> MAKEWGYASHNGPDHWHELFPNAKGENQSPIELHTKDIRHDPSLQPWSVSYDGGSAKTILNNGHTCNVVFDDTYDRSMLRGGPLPGPYRLRQFHLHWGSSDDHGSEHTVDGVKYAAELHLVHWNPKYNTFKEALKQRDGIAVIGIF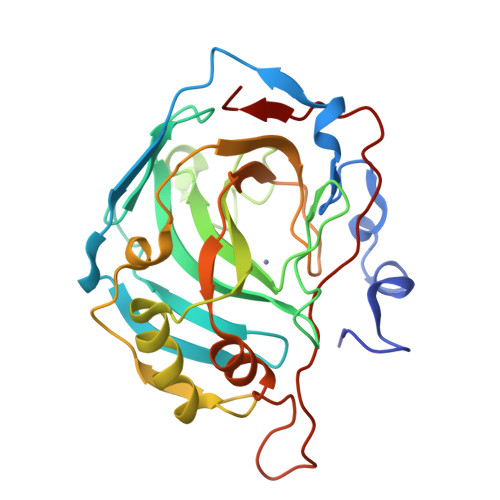LKIGHENGEFQIFLDALDKIKTKGKEAPFTKFDPSSLFPASRDYWTYQGSFTTPPCEECIVWLLLKEPMTVSSDQMAKLRSLLSSAENEPPVPLVSNWRPPQPINNRVVRASFK>MATYYYILASKKFLTEEEPLEEVFRERQRHYREQGKEIDFWLVPEPAFLEQPQFAEQKARCPQPAAAIISTNQQFIQWLKL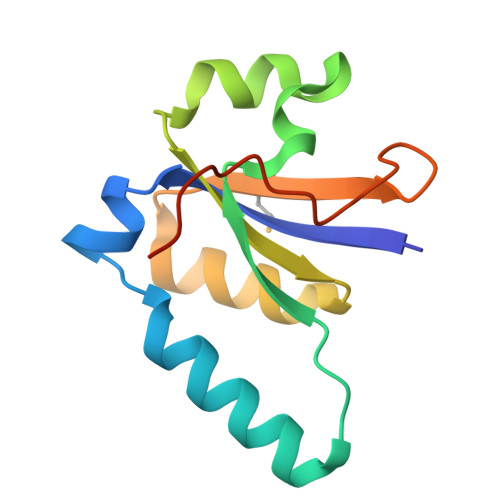RLEYVLMGQFTSEEVPNPLASLASVLEHHHHHH[6x]>[2x]MMHHH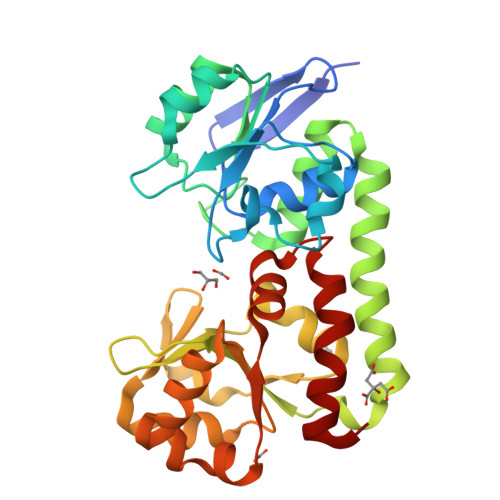HHHAVTITHLFGQTVIKEPPKRVVSAGYTEQDDLLAVDVVPIAVTDWFGDQPFAVWPWAAPKLGGARPAVLNLDNGIQIDRIAALKPDLIVAINAGVDADTYQQLSAIAPTVAQSGGDAFFEPWKDQARSIGQAVFAADRMRSLIEAVDQKFAAVAQRHPRWRGKKALLLQGRLWQGNVVATLAGWRTDFLNDMGLVIADSIKPFAVDQRGVIPRDHIKAVLDAADVLIWMTESPEDEKALLADPEIAASQATAQRRHIFTSKEQAGAIAFSSVLSYPVVAEQLPPQISQILGA>MHHHHHHTSLIEQPRWASKDSAAGAASTPDEKIVLEFMDALTSNDAAKLIEYFAEDTMYQNMPLPPAYGRDAVEQTLAGFFTVVSVDAVETFHIGSSNGLVYTERVDVLRALPTGKSYNFSILGVFQLTEGKITGWRDYFD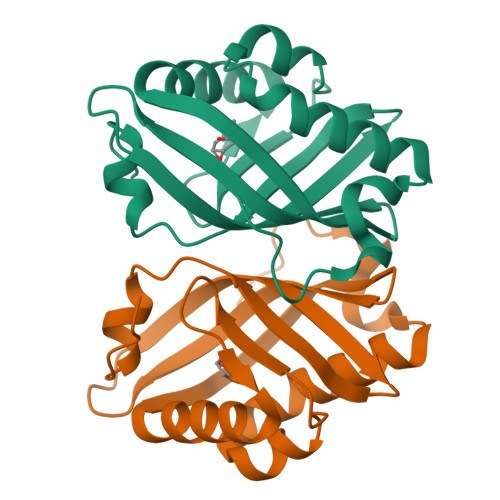LREFEEAVDLPLRG[8x]>[6x]MFEMIDSRTGVLNANDWKSQLRRSATTQALKKTTTNAEIILCNDESLKGLVQYDAFEKVTKLKRLPYWRSKGDANYYWADIDTTHVISH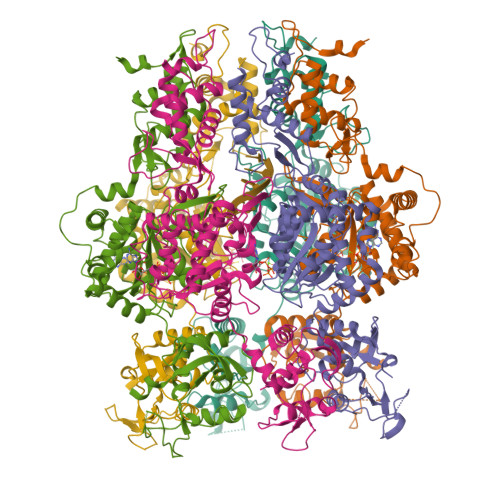IDKLYNVQFSRDLIDTVIEKEAYQNRFHPIKSMIESKSWDGIKRIETLFIDYLGAEDNHYNREVTKKWMMGAVARIYQPGIKYDSMIILYGGQGVGKSTAVSKLGGHWYNQSIKTFKGDEVYKKLQGSWICEIEELSAFQKSTIEDIKGFISAIVDIYRASYGKRTERHPRQCVFVGTTNNYEFLKDQTGNRRFFPITTDKNKATKSPFDDLTPVVVQQMFAEARVYFDENPTDKALLLDKEASEMALKVQEAHSEKDALVGEIEEFLERPIPSDYWYRTLEEKRVSAHDVIDQDYIKLYGDGKLIELPNAKPGAYVWRDKVCSMEIWKVMMKRDDQPQQHHLRKIDKALRNTNYCGTVKKQTRYGEGIGKQYGFSVDLASYYKNLKV> MSIDSALNWDGEMTVTRFDKMTGAHFVIRLDSTQLGPAAGGTRAAQYSQLADALTDAGKLAGAMTLKMAVSNLPMGGGKSVIALPAPRHSIDPSTWARILRIHAENIDKLSGNYWTGPDVNTNSADMDTLNDTTEFVFGRSLERGGAGSSAFTTAVGVFEAMKATVAHRGLGSLDGLTVLVQGLGAVGGSLASLAAEAGAQLLVADTDTERVAHAVALGHTAVALEDVLSTPCDVFAPCAMGGVITTEVARTLDCSVVAGAANNVIADEAASDILH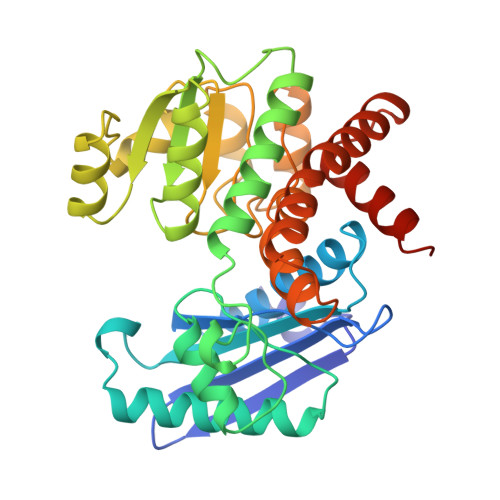ARGILYAPDFVANAGGAIHLVGREVLGWSESVVHERAVAIGDTLNQVFEISDNDGVTPDEAARTLAGRRAREASTTTATA> MEGWQRAFVLHSRPWSETSLMLDVFTEESGRVRLVAKGARSKRSTLKGALQPFTPLLLRFGGRGEVKTLRSAEAVSLALPLSGITLYSGLYINELLSRVLEYETRFSELFFDYLHCIQSLAGVTGTPEPALRRFELALLGHLGYGVNFTHCAGSGEPVDDTMTYRYREEKGFIASVVIDNKTFTGRQLKALNAREFPDADTLRAAKRFTRMA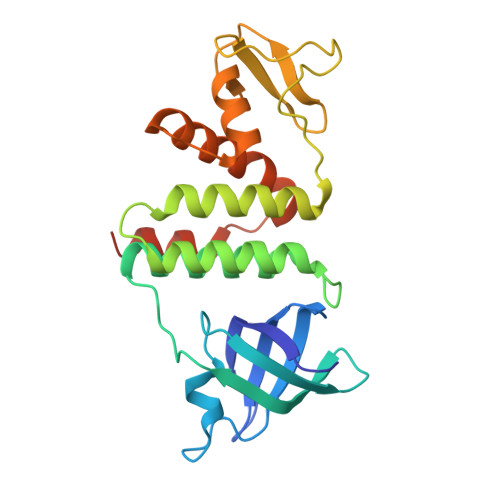LKPYLGGKPLKSRELFRQFMPKRTVKTHYE>[2x]PPLDLNNIQGDILGGLPKRTETYFFFDV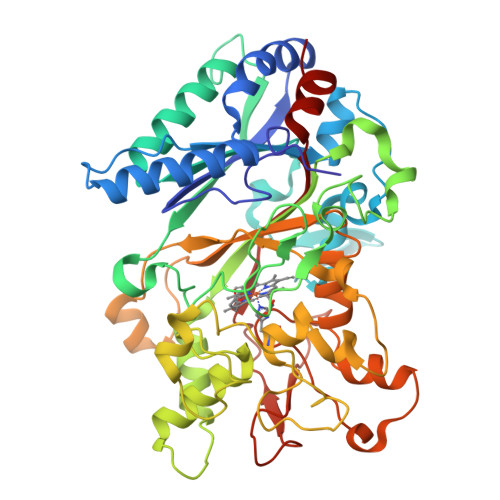TNVDQFKANMAHFIPHIKTSAGIIKDREAIKEHKRQKKPGLVPMAAVNVSFSHLGLQKLGITDDLSDNAFTTGQRKDAEILGDPGSKNGDAFTPAWEAPFLKDIHGVIFVAGDCHGSVNKKLDEIKHIFGVGTSHASISEVTHVRGDVRPGDVHAHEHFGWLDGISNPAVEQFDQNPLPGQDPIRPGFILAKENGDSRAAARPDWAKDGSFLTFRYLFQMVPEFDDFLESNPIVLPGLSRKEGSELLGARIVGRWKSGAPIEITPLKDDPKLAADAQRNNKFDFGDSLVRGDQTKCPFAAHIRKTYPRNDLEGPPLKADIDNRRIIRRGIQFGPEVTSQEHHDKKTHHGRGLLFVCYSSSIDDGFHFIQESWANAPNFPVNAVTSAGPIPPLDGVVPGFDAIIGQKVGGGIRQISGTNPNDPTTNITLPDQDFVVPRGGEYFFSPSITALKTKFAI> GKTNDWLDFDQLAEE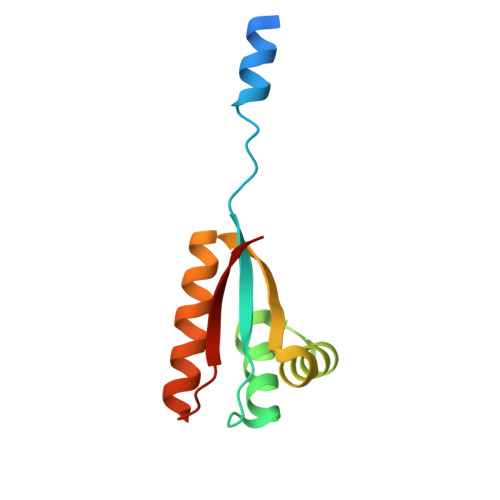KVRDALKPPSMYKVILVNDDYTPMEFVIDVLQKFFSYDVERATQLMLAVHYQGKAICGVFTAEVAETKVAMVNKYARENEHPLLCTLEKA>NEKFRPEMLQGKKVIVTGASKGIGREIAYHLAKMGAHVVVTARSKEALQKVVARCLELGAASAHYIAGSMEDMTFAEEFVAEAGNLMGGLDMLILNHVLYNRLTFFHGEIDNVRKSMEVNFHSFVVLSVAAMPMLMQSQGSIAVVSSVAGKITYPLIAPYSASKFALDGFFSTLRSEFLVNKVNVSITLCILGLIDTETAIKATSGIYLGPA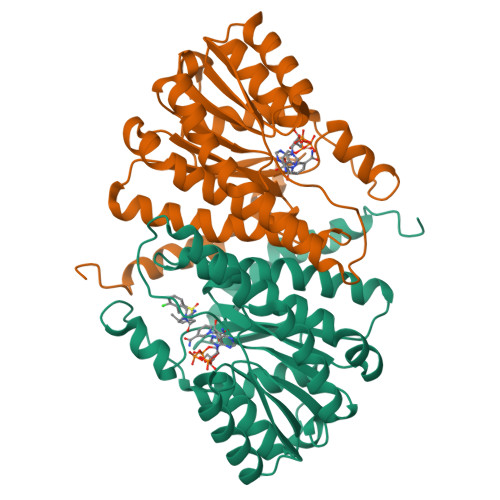SPKEECALEIIKGTALRQDEMYYVGSRWVPYLLGNPGRKIMEFLSAAEYNWDNVLSNEKLYGRWA[4x]>MSQHNILEALNVRVVGTGDRILFLAHGFGTDQSAWHLILPYFTQNYRVVLYDLVCAGSVNPDYFDFNR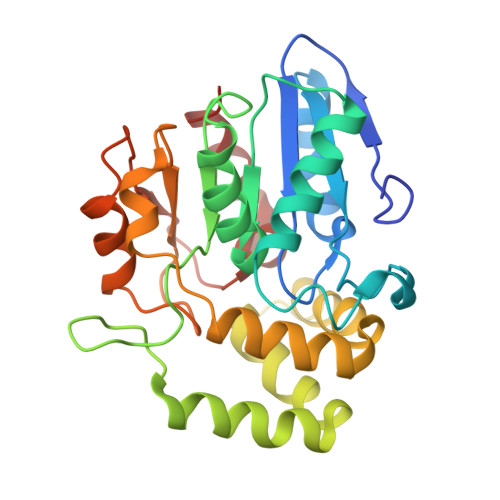YTTLDPYVDDLLNIVDSLGIQNCAYVGHSVSAMIGIIASIRRPELFSKLILIGFSPRFLNDEDYHGGFEEGEIEKVFSAMEANYEAWVHGFAPLAVGADVPAAVREFSRTLFNMRPDISLFVSRTVFNSDLRGVLGLVRVPTCVIQTAKDVSVPASVAEYLRSHLGGDTTVETLKTEGHLPQLSAPAQLAQFLRRALPR[4x]>[4x]SFIKPIYQDINSILIGQKVKRPKSGTLSGHAAGEPFEKLVYKFLKENLSDLTFKQYEYLNDLFMKNPAIIGHEARYKLFNSPTLLFLLSRGKAATENWSIENLFEEKQNDTADILLVKDQFYELLDVKTRNISKSAQAPNIISAYKLAQTCAKMIDNKEFDLFDINYLEVDWELNGEDLVCVSTSFAELFKSEPSELYINWAAAMQIQFHVRDLDQGFNGTREEWAKSYLK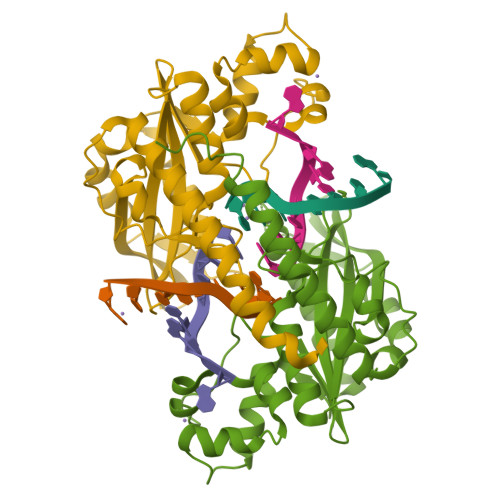HFVTQAEQRAISMIDKFVKPFKKYIL> QDLPTPPSVPTVHFHYFKLAVQPQVNKEIRNNNDINIDRTLVAKQSVVKFQLKTADLPAGRDETTSFVLVDPLPSGYQFNPEATKAASPGFDVTYDNATNTVTFKATAATLATFNADLTKSVATIYPTVVGQVLNDGATYKNNFTLTVNDAYGIKSNVVRVTTPGKPNDPDNPNNNYIKPTKVNKNENGVVIDGKTVLAGSTNYYELTWDLDQYK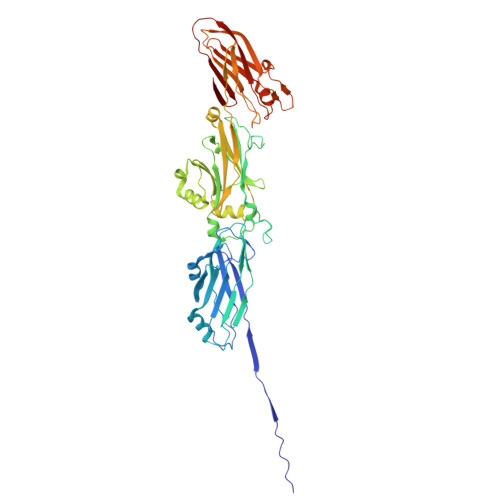NDRSSADTIQKGFYYVDDYPEEALELRQDLVKITDANGNEVTGVSVDNYTNLEAAPQEIRDVLSKAGIRPKGAFQIFRADNPREFYDTYVKTGIDLKIVSPMVVKKQMGQTGGSYENQAYQIDFGNGYASNIVINNVPKINPKKDVTLTLDPADTNNVDGQTIPLNTVFNYRLIGGIIPANHSEELFKYNFYDDYDQTGDHYTGQYKVFAKVDITLKNGVIIKSGTELTQYTTAEVDTTKGAITIKFKEAFLRSVSIDSAFQAESYIQMKRIAVGTFENTYINTVNGVTYSS>[4x]KGPNGLIERQV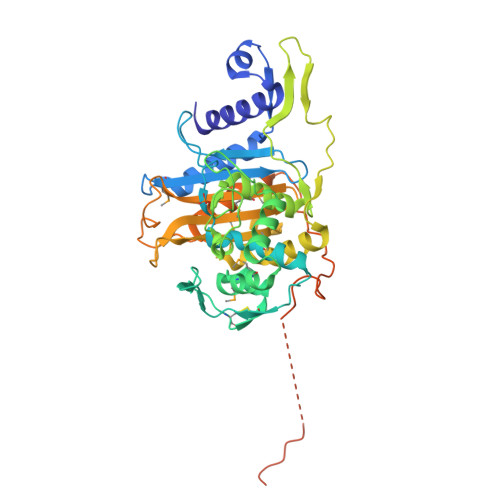TRELLELFNIDEQTLNTQGLVVTTTIDPQAQRAAEKAVAKYLDGQDPDMRAAVVSIDPHNGAVRAYYGGDNANGFDFAQAGLQTGSSFKVFALVAALEQGIGLGYQVDSSPLTVDGIKITNVEGEGCGTCNIAEALKMSLNTSYYRLMLKLNGGPQAVADAAHQAGIASSFPGVAHTLSEDGKGGPPNNGIVLGQYQTRVIDMASAYATLAASGIYHPPHFVQKVVSANGQVLFDASTADNTGDQRIPKAVADNVTAAMEPIAGYSRGHNLAGGRDSAAKTGTTQFGDTTANKDAWMVGYTPSLSTAVWVGTVKGDEPLVTASGAAIYGSGLPSDIWKATMDGALKGTSNETFPKPTEVGGYAGVPPPPPPPEVPPSETVIQPTVEIAPGITIPIGPPTTITLAPPPPAPPAATPTPPP> MAFNDLLKQVGGVGRFQLIQVTMVVAPLLLMASHNTLQNFTAAIPPHHCRPPANANLSKDGGLEAWLPLDKQGQPESCLRFTSPQWGPPFYNGTEANGTRVTEPCIDGWVYDNSTFPSTIVTEWNLVCSHRAFRQLAQSLYMVGVLLGAMVFGYLADRLGRRKVLILNYLQTAVSGTCAAYAPNYTVYCVFRLLSGMSLASIAINCMTLNVEWMPIHTRAYVGTLIGYVYSLGQFLLAGIAYAVPHWRHLQLVVSVPFF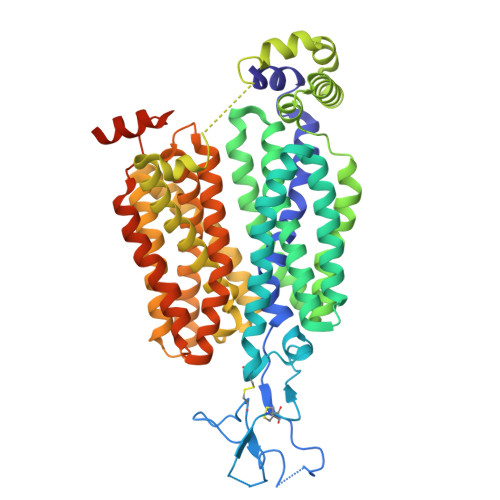IAFIYSWFFIESARWYSSSGRLDLTLRALQRVARINGKQEEGAKLSIEVLRTSLQKELTLSKGQASAMELLRCPTLRHLFLCLSMLWFATSFAYYGLVMDLQGFGVSMYLIQVIFGAVDLPAKFVCFLVINSMGRRPAQMASLLLAGICILVNGIIPKSHTIIRTSLAVLGKGCLASSFNCIFLYTGELYPTVIRQTGLGMGSTMARVGSIVSPLVSMTAEFYPSMPLFIFGAVPVVASAVTALLPETLGQPLPDTVQDLKSRSRGKQNQQQQEQQKQMMPLQASTQEKNGL Endo-β-N-acetylgucosaminidases (EC 3.2.1.96) (ENGases) are a class of enzymes that hydrolyze the glycosidic bond - GlcNAc β-1,4GlcNAc - present in N-linked sugar chains in glycoproteins and release the N-glycan moiety. Endo-A from Arthrobacter protophormiae is modular in architecture with three distinct domains. Domain 1, with residues 2–350 being identified, is the largest and displays a typical (β/α)8 TIM barrel fold, which has been observed for proteins belonging to family GH18 and GH20 of the glycoside hydrolases. Endo-A catalyses hydrolysis and transglycosylation via a substrate-assisted mechanism, in which the C2 acetamido group mounts a nucleophilic attack at the anomeric carbon resulting in the formation of an oxazoline ion intermediate.

Man3GlcNAc-thiazoline is an oxazoline mimic in which the anomeric oxygen at the reducing end was replaced with a sulfur atom. The Man3GlcNAc-thiazoline could be regarded as a transition state mimic and was resistant to Endo-A hydrolysis. The overall structures of the Endo-A in complex with Man3GlcNAc-thiazoline and Endo-A in complex with GlcNAc-Asn are identical to that of the free protein. While the thiazoline part of the carbohydrate moiety is buried deep inside a hydrophobic pocket formed by W93, F125, Y131, F169, Y205, F240, F243 and Y299, the mannose rings reside on the surface. As expected, the nitrogen atom of the thiazoline is hydrogen bonded to the side chain oxygen atom of N171. N171 probably orients the acetamido group for a nucleophilic attack and also stabilizes the transition states. Analysis of the structure of the binary complex of Endo-A with Man3GlcNAc-thiazoline reveals that E173 is well positioned to carry out the protonation of the anomeric carbon. The structure of Endo-A in complex with Man3GlcNAc-thiazoline reveals that N171 may be the essential residue that facilitates the intramolecular attack on GlcNAc during substrate assisted hydrolysis to form the 1,2-oxazoline ion intermediate. In the structures of the free Endo-A and Endo-A bound to Man3GlcNAc-thiazoline, the side chain of W244 is perpendicular to W216 and introduces a steric block at the entrance of the active site.

>[4x]STYNGPLSSHWFPEELAQWEPDSDPDAPFNRSHVPLEPGRVADRVNANADKDAHLVSLSALNRHTSGVPSQGAPVFYENTFSYWHYTDLMVYWAGSAGEGIIVPPSADVIDASHRNGVPILGNVFFPPTVYGGQLEWLEQMLEQEEDGSFPLADKLLEVADYYGFDGWFINQETEGADEGTAEAMQAFLVYLQEQKPEGMHIMWYDSMIDTGAIAWQNHLTDRNKMYLQNGSTRVADSMFLNFWWRDQRQSNELAQALGRSPYDLYAGVDVEARGTSTPVQWEGLFPEGEKAHTSLGLYRPDWAFQSSETMEAFYEKELQFWVGSTGNPAETDGQSNWPGMAHWFPAKSTATSVPFVTHFNTGSGAQFSAEGKTVSEQEWNNRSLQDVLPTWRWIQHGGDLEATFSWEEAFEGGSSLQWHGSLAEGEHAQIELYQTELPISEGTSLTWTFKSEHDNDLNVGFRLDGEEDFRYVEGEQRESINGWTQWTLPLDAFAGQTITGLAFAAEGNETGLAEFYTGQLAVGADSEKPAAPNVNVRQYDPDPSGIQLVWEKQSNVHHYRVYKETKHGKELIGTSAGDRIYIEGLVEESKQNDVRLHIEALSETFVPSDARMIDIKSGSF> MKTICLVGGKLQGFEAAYLSKKAGMKVVLVDKNPQALIRNYADEFYCFDVIKEPEKLLELSKRVDAVLPVNENLACIEFLNSIKEKFSCPVLFDFEAYRISRDKKKSKDYFKSIGVPTPQDRPSKPPYFVKPPCESSSVGARIIYDDKDLEGLEPDTLVEEYVEGEVVSLEVVGDGSHFAVVKETLVHIDETYDCHMVTPLPANPLFRQISHD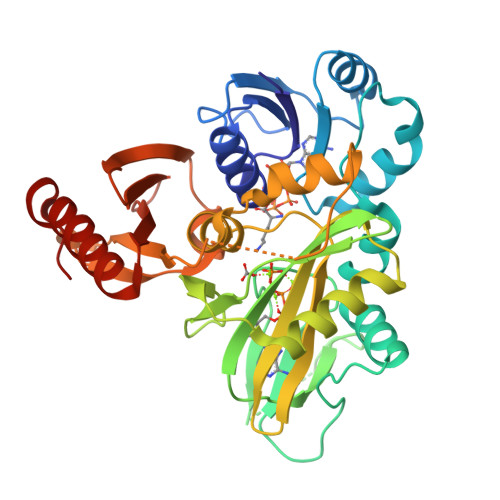LAANLPLKGIMDVEAIFGPKGLRVIEIDARFPSQTPTVVYYSSGINLIELLFRAFTDGVEEIRAIPENKYCIYEHLMFGENGVLIPVGEQVLSMGSDYGKFYEEPGIEIFLCKGEYPVFTMVFWGKDREETGAKRCKGLSVLKERFGAVL(E)-(2R,3R,4S,5R)-3,4,5-TRIHYDROXY-2-METHOXY-8,8-DIMETHYL-NON-6-ENOIC ACID ((3S,6R)-6-HYDROXY-2-OXO-AZEPAN-3-YL)-AMIDE 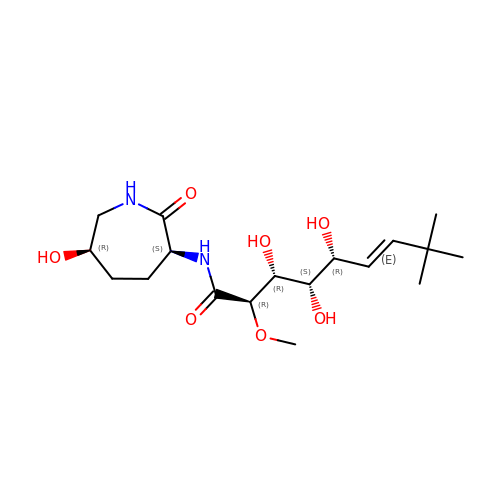| C18 H32 N2 O7 | FVBBTOIQETYGOA-SDNORSGYSA-N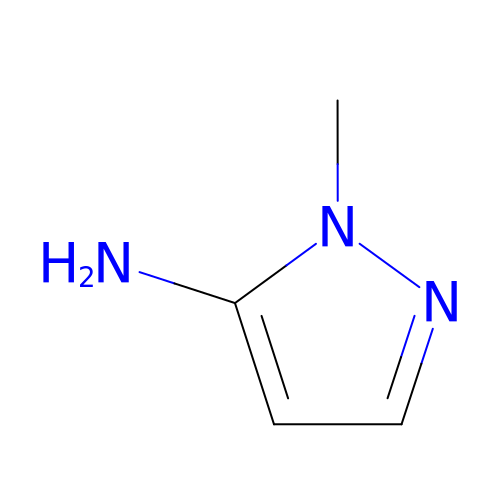1-methyl-1H-pyrazol-5-amine | C4 H7 N3 | JESRNIJXVIFVOV-UHFFFAOYSA-N2-[(5-hex-1-yn-1-ylfuran-2-yl)carbonyl]-N-methylhydrazinecarbothioamide 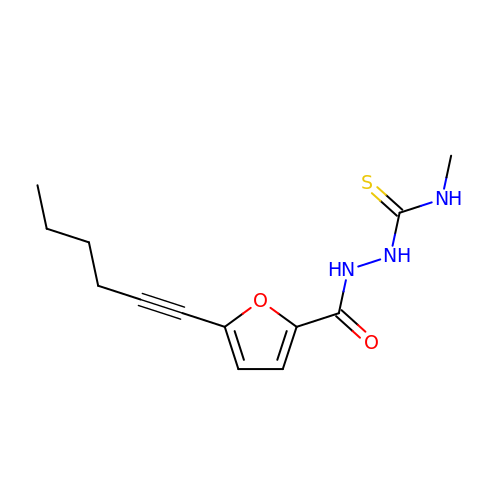| C13 H17 N3 O2 S | CUKZXTKQBXLMDO-UHFFFAOYSA-N> RSVAETPTYPWRDAETGERLVCAQCPPGTFVQRPCRRDSPTTCGPCPPRHYTQFWNYLERCRYCNVLCGEREEEARACHATHNRACRCRTGFFAHAGFCLEHASCPPGAGVIAPGTPSQNTQCQPCPPGTFSASSSSSEQCQPHRNCTALGL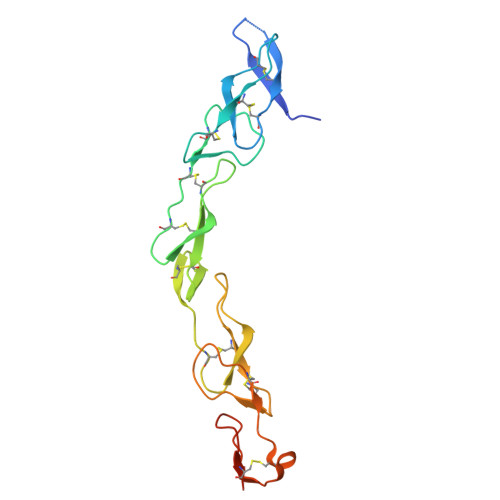ALNVPGSSSHDTLCTSTGHHHHHH4-[8-azanyl-3-[(3~{R})-1-(3-methyloxetan-3-yl)carbonylpiperidin-3-yl]imidazo[1,5-a]pyrazin-1-yl]-~{N}-[4-(trifluoromethyl)pyridin-2-yl]benzamide | C29 H28 F3 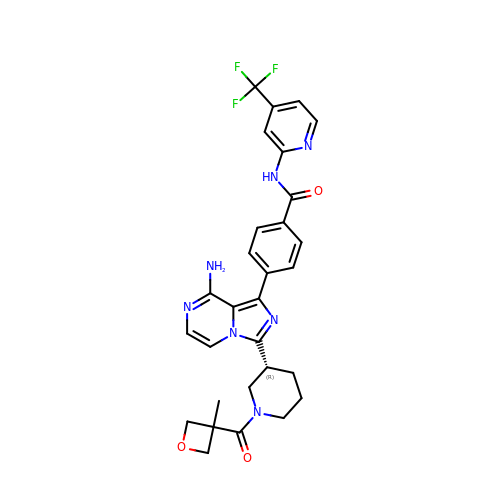N7 O3 | AHBFBRPGNOVEBK-LJQANCHMSA-N> 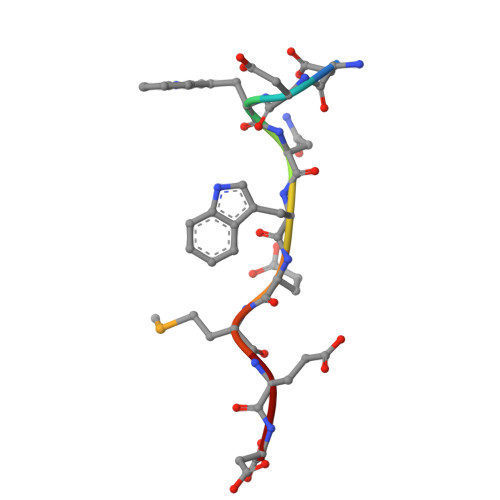DDWNWEMED>GSHMQEESRCQRCISELKDIRLQLEACETRTVHRLRLPLDKEPARECAQRIAEQQKAQAEVEGLGKGVARLSAEAEKVLALPEPSPAAPTLRSELELTLGKLEQVRSLSAIYLEKLKTISLVIRGTQGAEEVLRAHEEQLKEAQAVPATLPELEATKASLKKLRAQAEAQQPTFDALRDELRGAQEVGERLQQRHGERDVEVERWRER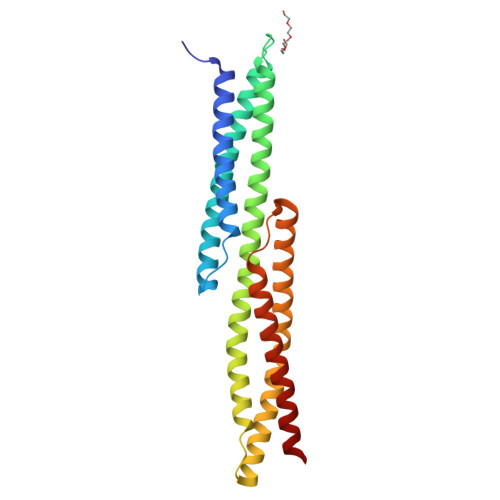VAQLLERWQAVLAQTDVRQRELEQLG[2x]>MKCPVCHQGEMVSGIKDIPYTFRGRKTVLKGIHGLYCVHCEESIMNKEE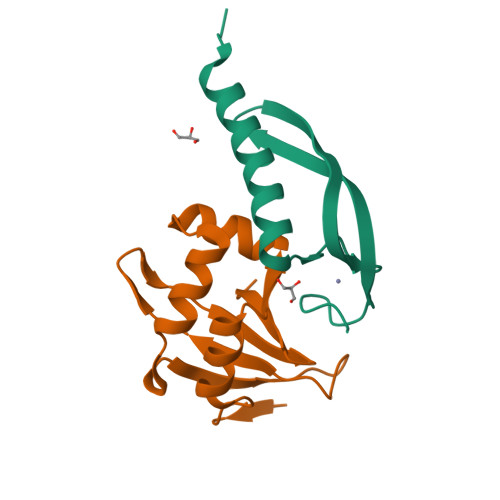SDAFMAQVKAFRASVNAETVAPEFIVK[2x];>[2x]GSHMEKRTPHTRLSQVKKLVNAGQVRTTRSALLNADELGLDFDGMCNVIIGLSESDFYKSMTTYSDHTIWQDVYRPRLVTGQVYLKITVIHDVLIVSFKEK Haloalkane dehalogenases (HLDs) are α/β-hydrolase fold enzymes that catalyse the cleavage of carbon–halogen bonds in halogenated compounds through an SN2 nucleophilic substitution mechanism, producing a corresponding alcohol, a halide and a proton. Recently, database-mining searches identified a new haloalkane dehalogenase, DmmarA, encoded in the genome of the waterborne pathogenic bacterium Mycobacterium marinum M. This bacterium causes a tuberculosis-like illness in fish and can lead to infections in humans, particularly those with immune deficiencies. However, DmmarA differs from the other members of the HLD-II subfamily as it contains an aspartic acid instead of a glutamic acid as the catalytic acid in the catalytic triad. The overall structure of DmmarA shows a canonical HLD fold that shares major structural features with other HLDs.

Crystallization screening and subsequent crystal-growth optimization identified two chemical conditions, at pH 6.5 and pH 5.5, where we could reproducibly obtain DmmarA crystals. The first structure originated from a crystal grown in mother liquor composed of 0.02 M KH2PO4, 0.1 M bis-Tris propane pH 6.5, 22% PEG 3350. This crystal structure was solved to a resolution of 1.85 Å in space group P1211, with unit-cell parameters a = 91.816, b = 61.381, c = 106.689 Å, α = 90, β = 106.256, γ = 90°. The Matthews Probability Calculator suggested four DmmarA (∼33 000 Da) molecules in the asymmetric unit and these were identified in molecular-replacement searches. The asymmetric units of both crystal forms of DmmarA (pH 6.5 and pH 5.5) contain four protein chains (A–D), of which chains A and B form the first biological homodimer and chains C and D form the second biological dimer. The active site of DmmarA is located between the main α/β-core and the helical cap domain. In the active site we find the proton-relay catalytic triad, which is atypically composed of a nucleophilic aspartate (Asp95), a base histidine (His259) and a catalytic acid (Asp119). Careful inspection of the electron-density maps revealed an atypical mode of DmmarA homodimerization that has not previously been observed. Precisely, the DmmarA structure displays a new so-called back-to-back homodimerization mode, distinguishing it from the previously described HLD dimers. The DmmarA homodimer is assembled due to noncovalent interactions between the L5 loop located in the main α/β-core, the α5′ and α7 helices in the cap domain of one chain and the corresponding symmetric interface of the second chain. Our crystallographic analysis, supported by nanoDSF and SAXS experiments, provides evidence that the DmmarA enzyme forms symmetric homodimers, predominantly due to the specific composition and conformation of the L5 loop.

>[4x]MKRVDVLDSAMSYIDVGQGDPIVFLHGNPTSSYLWRNVIPHLSDVGRCLAPDLIGMGASGTSPTFSYRFADHVRYLDAWFEAVGITENVVLVVHDWGSALGFYRALRYPEQIAGIAYMDALVQPRTWAGFTDYEPLMRALRTEQGERMALAENVFVEKVVPGGVQRQLTEEEMAVYRTPYPTPQSRIPTLLWAREIPVEGEPADVQAMVQEYADFLSRSDIPKLLIVAEPGAILHEGGSELDFARSWPNQREVKVAGRHFLQEDSPDAIGAAVRAFVLDVRERQDGADRAHHHHHH> PISPIETVPVKLKPGMDGPKVKQWPLTEEKIKALVEICTEMEKEGKISKIGPENPYNTPVFAIKKKDSTKWRKLVDFRELNKRTQDFWEVQLGIPHPAGLKKKKSVTVLDVGDAYFSVPLDEDFRKYTAFTIPSINNETPGIRYQYNVLPQGWKGSPAIFQSSMTKILEPFKKQNPDIVIYQYMDDLYVGSDLEIGQHRTKIEELRQHLLRWGLTTPDKKHQKEPPFLWMGYELHPDKWTVQPIVLPEKDSWTVNDIQKLVGKLNWASQIYPGIKVRQLCKLLRGTKALTEVIPLTEEAELELAENREILKEPVHGVYYDPSKDLIAEIQKQGQGQWTYQIYQE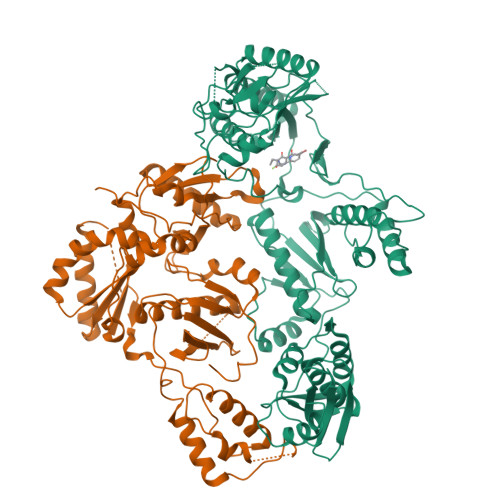PFKNLKTGKYARMRGAHTNDVKQLTEAVQKITTESIVIWGKTPKFKLPIQKETWETWWTEYWQATWIPEWEFVNTPPLVKLWYQLEKEPIVGAETFYVDGAANRETKLGKAGYVTNKGRQKVVPLTNTTNQKTQLQAIYLALQDSGLEVNIVTDSQYALGIIQAQPDKSESELVNQIIEQLIKKEKVYLAWVPAHKGIGGNEQVDKLVSAGIR;> PISPIETVPVKLKPGMDGPKVKQWPLTEEKIKALVEICTEMEKEGKISKIGPENPYNTPVFAIKKKDSTKWRKLVDFRELNKRTQDFWEVQLGIPHPAGLKKKKSVTVLDVGDAYFSVPLDEDFRKYTAFTIPSINNETPGIRYQYNVLPQGWKGSPAIFQSSMTKILEPFKKQNPDIVIYQYMDDLYVGSDLEIGQHRTKIEELRQHLLRWGLTTPDKKHQKEPPFLWMGYELHPDKWTVQPIVLPEKDSWTVNDIQKLVGKLNWASQIYPGIKVRQLCKLLRGTKALTEVIPLTEEAELELAENREILKEPVHGVYYDPSKDLIAEIQKQGQGQWTYQIYQEPFKNLKTGKYARMRGAHTNDVKQLTEAVQKITTESIVIWGKTPKFKLPIQKETWETWWTEYWQATWIPEWEFVNTPPLVKLWY> GSDDGAFGDIWAYMSEALTGAPGKIIACGMLFSVAYFGVVKPNLGLALVSALMMLVMANGEKIISSFLRAGI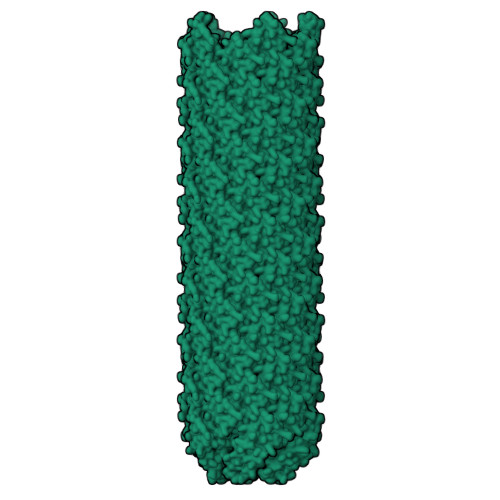PL>MILSVHILDQQTGKPAPGVEVVLEQKKDNGWTQLNTGHTDQDGRIKALWPEKAAAPGDYRVIFKTGQYFESKKL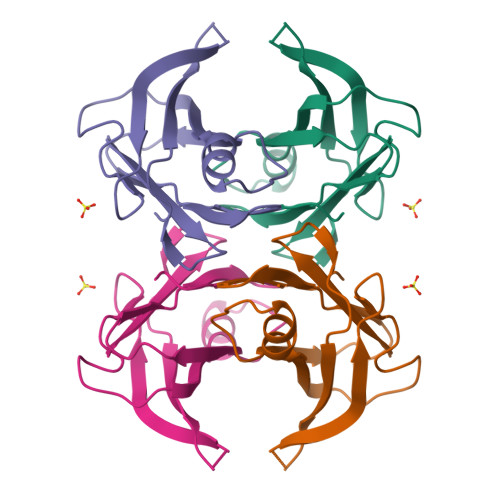DTFFPEIPVEFHISKTNEHYHVPLLLSQYGYSTYRGS[2x]>MPEHNRRLVERTGIDVEKLLELLIKAAAAEFTTYYYYTILRNHATGLEGEAIKEIIEDARLEDRNHFEALVPRIYELGGELPRDIREFADLASCRDAYLPEEPTIENILKVLLEAERCAVGVYTEICNYTFGKDPRTYDLALAILHEEIEHEAWFEELLTGKPSGHFRRGKPGESPYVSKFLKTR[12x]

The ferritin protein superfamily, nearly ubiquitous throughout the tree of life, has evolved to address iron storage, iron toxicity and free radical formation. ,, Ferritins oxidize Fe­(II) to Fe­(III) and store it within the ferritin nanoparticle as hydrated ferric oxyhydroxide. First identified in hyperthermophilic archaea, DPSL forms a 12-subunit (dodecameric) nanocage that preferentially utilizes H2O2 as a substrate. ,,, For these reasons, DPSL was first perceived as a DPS-Like mini-ferritin. However, structural studies revealed a surprise; DPSL lacks the DPS ferroxidase site and instead retains a bacterioferritin-like ferroxidase center in the middle of the 4-helix bundle. For these reasons, DPSL is proposed to lie at the evolutionary interface between the mini- and maxi-ferritins. ,− Importantly, DPSL further differentiates itself from both the (bacterio)­ferritins and DPS by the presence of two conserved cysteine residues that are juxtaposed between the ferroxidase center and the exterior surface of the particle. Together, the conserved cysteines and the bacterioferritin-like ferroxidase center serve as hallmarks of the archaeal DPSL proteins that are easily identified within the sequence as a “thioferritin” motif, and serve to differentiate DPSL as a distinct member of the ferritin superfamily.

Further, if the mineral is indeed present as ferrihydrite, it also suggests a 3-fold axis in ferrihydrite (space group P63mc) should align coincident with a 3-fold axis in Pf-DPSL; and that if particles with a single crystallite could be identified, a C3 reconstruction might indeed resolve the mineral structure. To test this hypothesis, and because the 3-fold pores in DPSL are related to each other by D2 symmetry, the iron loaded data set was D2 symmetry expanded. Masks covering the densest mineral features coordinated by residues 168–171 at each of the four positions were then constructed and used to sort for the presence of mineral at the first site (lying on the z axis), but the absence of mineral at the remaining three sites. This identified 167,240 particles with significant iron density at a single 3-fold. Homogenous refinement with 3-fold (C3) symmetry then gave a map with strong mineral density for the C-terminal coordinated mineral along the Z axis. While the overall resolution of this map was 2.5 Å, the mineral is significantly less ordered. Nevertheless, there was clearly resolved density for a constellation of 4 iron atoms with tetrahedral geometry centered on the 3-fold axis. The density is proximal to residues 168–171 and highly similar to the 4Fe/4O cluster in the ferrihydrite structure of Michel et al. Further, when the Michel ferrihydrite crystal structure was symmetry expanded and superpositioned upon the modeled irons, we identified an extended ferrihydrite superstructure with 13 Fe and 18 O atoms that was consistent with the surrounding density.>VVKEEGFARGADVSWLTQMEAEGLKFYTPDENRQEMECMDLLRDYCGVNSIRLRVWVNPKDGWNNMNDVIVKAKRAERLGLR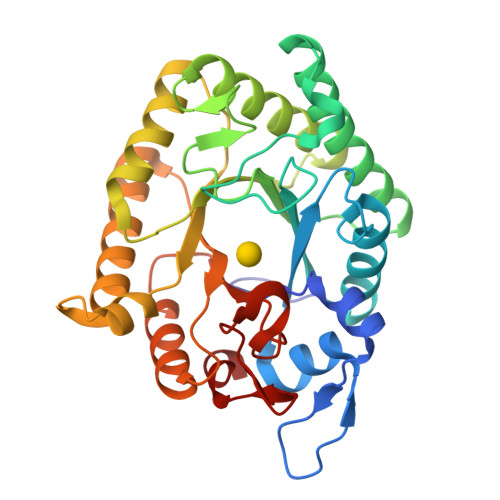TMIDFHFSDTWADPGHQEMPEAWKELSFDDLKIALSEHVKSVLTALKAVGVTPEWVQVGNETTPGMMLPVGSVDNPEQLTALNNAGYDAVKAICPDAKVIVHLDAGNDQWVYNRMFDILQANGGKYDMIGMSLYPYWAEQEGKTGGWLKVADDCIANIKHVKQKYNKPVMICEIGMPYDQAEACKQLITKMMQADVEGIFYWEPQAPNGYNDGYNLGCFDNNAPTIALDAFK[2x]Methylation of cytosine 32 in the anticodon loop of tRNAs to 3-methylcytosine (m3C) is crucial for cellular translation fidelity. Here, we report the cryo-electron microscopy structure of the human m3C tRNA methyltransferase METTL6 in complex with seryl-tRNA synthetase (SerRS) and their common substrate tRNASer. We show that SerRS acts as the tRNASer substrate selection factor for METTL6. We demonstrate that SerRS augments the methylation activity of METTL6 and that direct contacts between METTL6 and SerRS are necessary for efficient tRNASer methylation.

Despite attempts to crystallize the complex, we could only achieve two crystal forms of METTL6 bound to SAH and the complex disintegrated during cryo-EM grid preparation. To determine whether tRNA binding to METTL6 induces conformational changes in the enzyme, we compared our structural model to the crystal structures of METTL6 bound to either SAM or SAH, but without an RNA ligand. The methyltransferase core of all models aligns well. Deviations occur exclusively in the m3C-RBD, in particular in the divergent N-terminal region, the substrate-binding loop and the β-extension. All RNA-free structures display disordered substrate-binding loops, which seem to adopt their shape only in contact with the tRNA, and a conserved helix following the substrate-binding loop is rearranged on interaction with the ligand. Our data suggest some degree of flexibility in the region of the β-extension hairpin, a region that is completely unresolved in the crystal structures, suggesting its plasticity for tRNASer accommodation. Thus, while the core of METTL6 is rigid, parts of the m3C-RBD seem to be more ductile, to accommodate the tRNA.

>[2x]GPDSMEAQKNWDLFYKRNSTNFFKDRHWTTREFEELRSCREFEDQKLTMLEAGCGVGNCLFPLLEEDPNIFAYACDFSPRAIEYVKQNPLYDTERCKVFQCDLTKDDLLDHVPPESVDVVMLIFVLSAVHPDKMHLVLQNIYKVLKPGKSVLFRDYGLYDHAMLRFKASSKLGENFYVRQDGTRSYFFTDDFLAQLFMDTGYEEVVNEYVFRETVNKKEGLCVPRVFLQSKFLKP1-[8-(2,5-dimethoxyphenyl)pyrrolo[1,2-a]pyrimidin-6-yl]ethanone | C17 H16 N2 O3 | 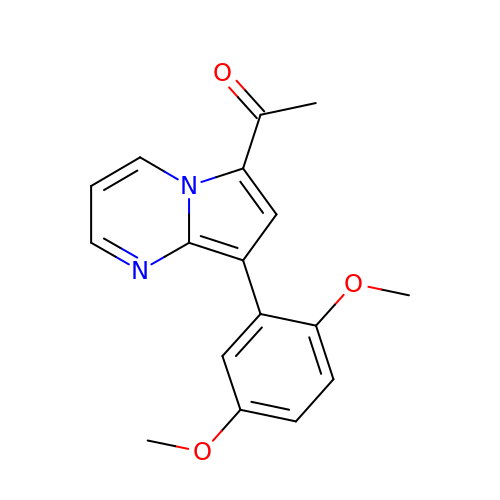VNCOLZXZXMUDIT-UHFFFAOYSA-N>MAYQTIYPYTNEVLHTFDNMTDQGLADVLERAHLLYKKWRKEDHLEERKAQLHQVANILRRDRDKYAEIMTKDMGKLFTEAQGEVDLCADIADYYADKADEFLMSTPLETDSGQAYYLKQSTGVILAVEPWNFPYYQIMRVFAPNFIVGNPMVLKHASICPRSAQSFEELVLEAGAEAGSITNLFISYDQVSQVIADKRVVGVCLTGSERGGASIAEEAGKNLKKTTLELGGDDAFIILDDADWDQLEKVLYFSRLYNAGQVCTSSKRFIVLDKDYDRFKELLTKVFKTAKWGDPMDPETTLAPLSSAQAKADVLDQIKLALDHGAELVYGGEAIDHPGHFVMPTIIAGLTKDNPIYYQEIFGPVGEIYKVSSEEEAIEVANDSNYGLGGTIFSSNQEHAKAVAAKIETGMSFINSGWTSL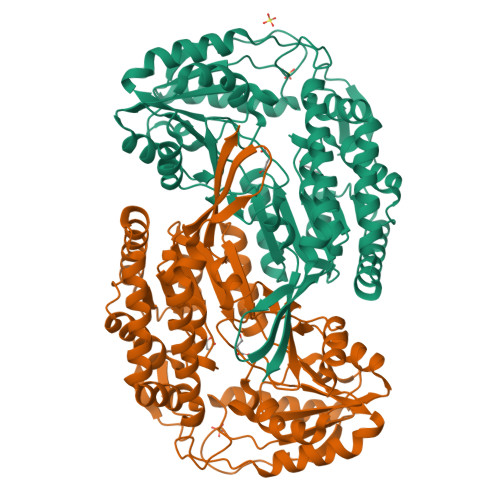PELPFGGIKHSGYGRELSELGFTSFVNEHLIYIPNKTNNSNTKV[2x]~{N}-[[(3~{S})-1-ethanoylpyrrolidin-3-yl]methyl]-~{N}-methyl-4-quinolin-7-yl-benzenesulfonamide | C23 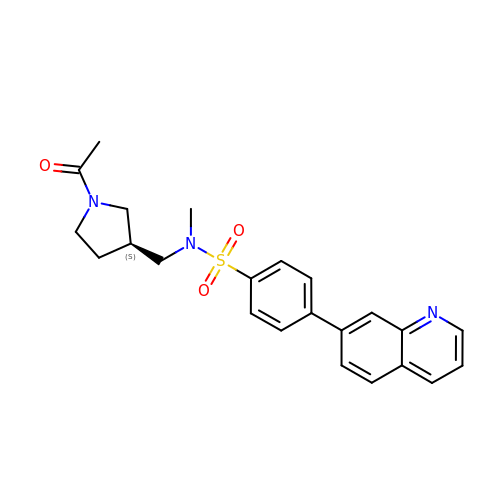H25 N3 O3 S | ODJLDVQUQRRAAY-GOSISDBHSA-N>GSHMATPWSGYLDDVSAKFDTGVDNLQTQVTEALDKLAAKPSDPALLAAYQSKLSEYNLYRNAQSNTVKVFKDIDAAIIQNFRGGSGGTTISDAEIWDMVSQNISAIGDSYLGVYENVVAVYTDFYQAFSDILSKMGGWLLPGKDGNTVKLDVTSLKNDLNSLVNKYNQINSNTVLFPAQSGSGVKVATEAEARQWLSELNLPNSCLKSYGSGYVVTVDLTPLQKMVQDIDGLGAPGKDSKLEMDNAKYQAWQSGFKAQEENMKTTLQTLTQKYSNANSLYD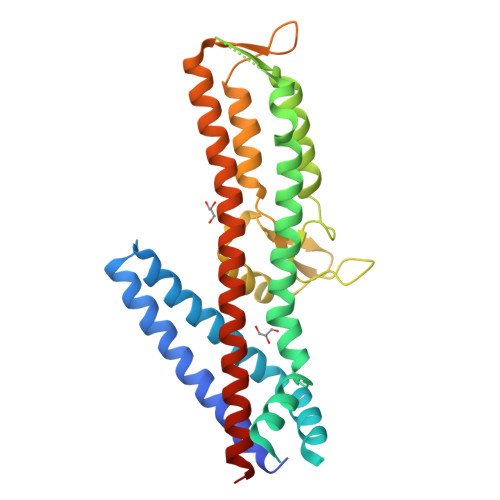NLVKVLSSTISSSLETAKSFLQG[2x]> MDEATWERMWKHVAKIHPDGEKVAQRIRGATDLPKIPIPSVPTFQPSTPVPERLEAVQRYIRELQYNHTGTQFFEIKKSRPLTGLMDLAKEMTKEALPIKCLEAVILGIYLTNSMPTLERFPISFKTYFSGNYFRHIVLGVNFAGRYGALGMSRREDLMYKPPAFRTLSELVLDFEAAYGRCWH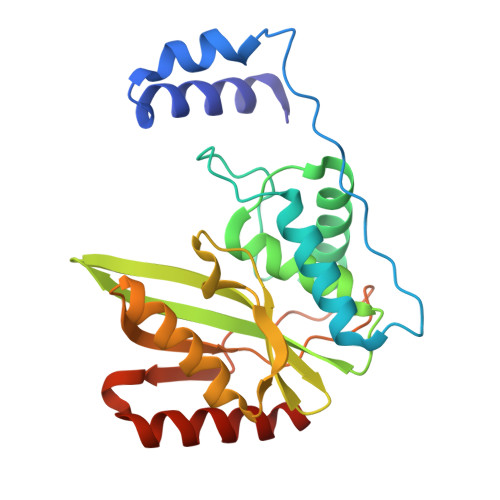VLKKVKLGQSVSHDPHSVEQIEWKHSVLDVERLGRDDFRKELERHARDMRLKIG>[2x]GSGAPPTDLQKMVMGNTKPVELILDGKTVAICCATGVFGTAYLVPRHLFAEKYDKIMLDGRAMT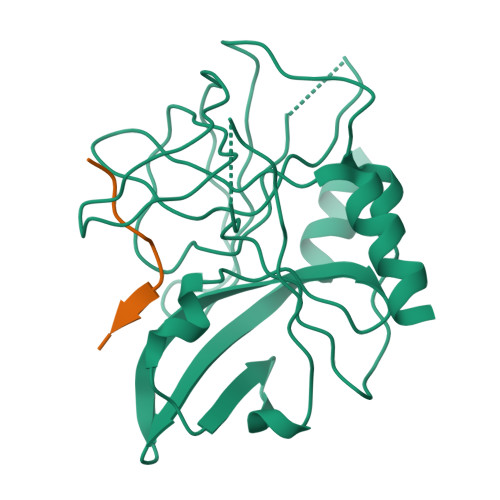DSDYRVFEFEIKVKGQDMLSDAALMVLHRGNKVRDITKHFRDTARMKKGTPVVGVVNNADVGRLIFSGEALTYKDIVVLMDGDTMPGLFAYKAATRAGYAGGAVLAKDGADTFIVGTHSAGGNGVGYCSCVSRSMLQKMKAHVDPEPHHE;>[2x]XAPAKQLLNFD>MLNPIVRKFQYGQHTVTLETGMMARQATAAVMVSMDDTAVFVTVVGQKKAKPGQDFFPLTVNYQERTYAAGRIPGSFFRREGRPSEGETLIARLIDRPIRPLFPEGFVNEVQVIATVVSVNPQVNPDIVAMIGASAALSLSGIPFNGPIGAARVGYINDQYVLNPTQDELKESKLDLVVAGTEAAVLMVESEAQLLSEDQMLGAVVFGHEQQQVVIQNINELVKEAGKPRWDWQPEPVNEALNARVAALAEARLSDAYRITDKQERYAQVDVIKSETIATLLAEDETLDENELGEILHAIEKNVVRSRVLAGEPRIDGREKDMIRGLDVRTGVLPRTHGSALFTRGETQALVTATLGTARDAQVLDELMGERTDTFLFHYNFPPYSVGETGMVGSPKRREIGHGRLAKRGVLAVMPDMDKFPYTVRVVSEITESNGSSSMASVCGASLALMDAGVPIKAAVAGIAMGLVKEGDNYVVLSDILGDEDHLGDMDFKVAGSRDGISALQMDIKIEGITKEIMQVALNQAKGARLHILGVMEQAINAPRGDISEFAPRIHTIKINPDKIKDVIGKGGSVIRALTEETGTTIEIEDDGTVKIAATDGEKAKHAIRRIEEITAEIEVGRVYTGKVTRIVDFGAFVAIGG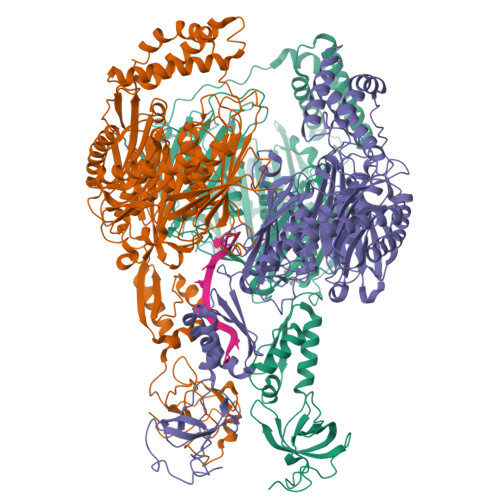GKEGLVHISQIADKRVEKVTDYLQMGQEVPVKVLEVDRQGRIRLSIKEATEQSQPAAAPEAPAAEQGE[3x]> DQAGKSPNAVRYHGGDEIILQGFHWNVVREAPNDWYNILRQQAATIAADGFSAIWMPVPWRDFSSWSDGSKSGGGEGYFWHDFNKNGRYGSDAQLRQAASALGGAGVKVLYDVVPNHMNRGYPDKEINLPAGQGFWRNDCADPGNYPNDCDDGDRFIGGDADLNTGHPQVYGMFRDEFTNLRSQYGAGGFRFDFVRGYAPERVNSWMTDSADNSFCVGELWKGPSEYPNWDWRNTASWQQIIKDWSDRAKCPVFDFALKERMQNGSIADWKHGLNGNPDPRWREVAVTFVDNHDTGYSPGQNGGQHHWALQDGLIRQAYAYILTSPGTPVVYWDHMYDWGYGDFIRQLIQVRRAAGVRADSAISFHSGYSGLVATVSGSQQTLVVALNSDLGNPGQVASGSFSEAVNASNGQVRVWRSGTGSGGGEPGALVSVSFRCDNGATQMGDSVYAVGNVSQLGNWSPAAALRLTDTSGYPTWKGSIALPAGQNEE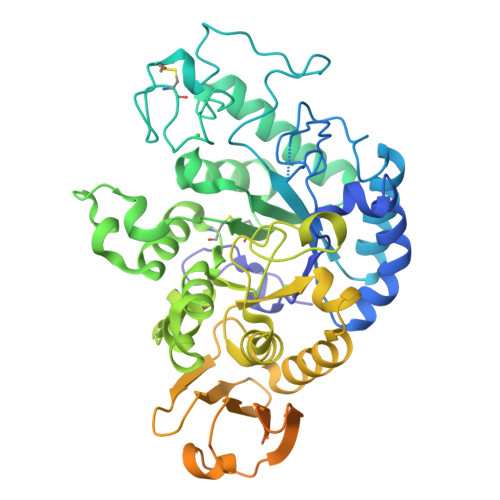WKCLIRNEANATQVRQWQGGANNSLTPSEGATTVGRL>GAINKNMKLGQKVLIPVKQFPKFNFVGKLLGPRGNSLKRLQEETLTKMSILGKGSMRDKAKEEELRKSGEAKYFHLNDDLHVL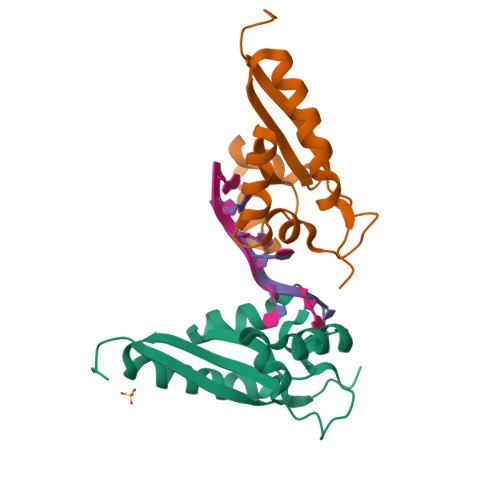IEVFAPPAEAYARMGHALEEIKKFLIPDYN[6x]> GLTIPKAVQYLSSQDEKYQAIGAYYIQHTCFQDESAKQQVYQLGGICKLVDLLRSPNQNVQQAAAGALRNLVFRSTTNKLETRRQNGIREAVSLLRRTGNAEIQKQLTGLLWNLSSTDELKEELIADALPVLADRVIIPFSGWCDGNSNMSREVVDPEVFFNATGCLRNLSSADAGRQTMRNYSGLIDSLMAYVQNCVAASRCDDKSVENCMCVLHNLSYRLDAEVPTRYRQLEYNARNAYTEKSSTGCFSNKSDKMMNNNYDCPLPEEETNPKGSGWLYHSDAIRTYLNLMGKSKKDATLEACAGALQNLTASKGLMSSGMSQLIGLKEKGLPQIARLLQSGNSDVVRSGASLLSNMSR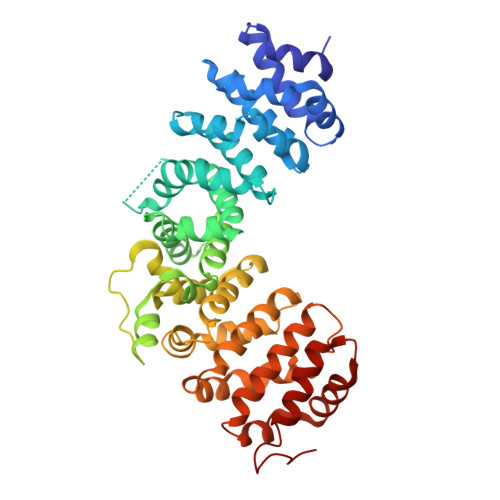HPLLHRVMGNQVFPEVTRLLTSHTGNTSNSEDILSSACYTVRNLMASQPQLAKQYFSSSMLNNIINLCRSSASPKAAEAARLLLSDMWSSKELQGVL N-methyl-D-aspartic acid | C5 H9 N O4 | 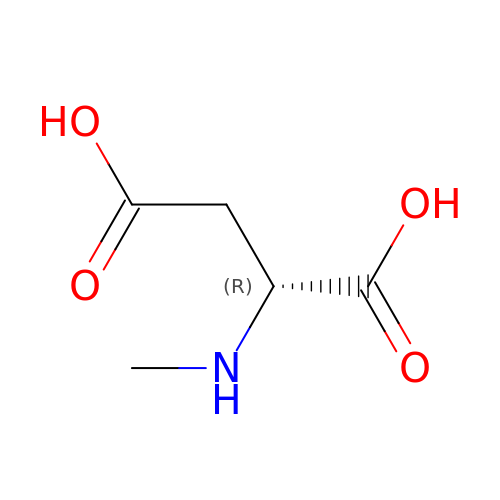HOKKHZGPKSLGJE-GSVOUGTGSA-N>GGSMSKTIVLSVG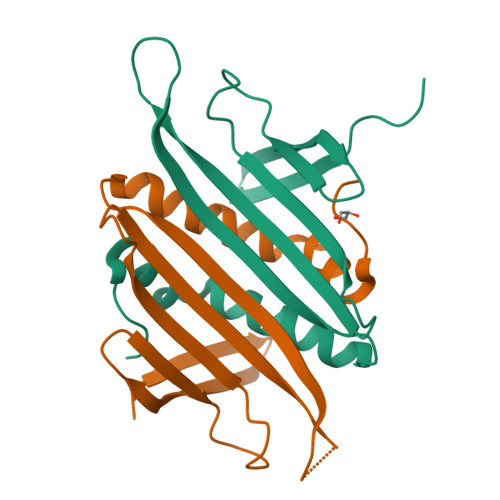EATRTLTEIQSTADRQIFEEKVGPLVGRLRLTASLRQNGAKTAYRVNLKLDQADVVDSGLPKVRYTQVWSHDVTIVANSTEASRKSLYDLTKSLVATSQVEDLVVNLVPLGR[2x]The prototypical systems used to study sequential RNA assembly are group II introns, another class of highly-conserved self-splicing ribozymes of biomedical and bioengineering relevance. Group II introns are validated drug targets for antifungal antibiotics, potentially powerful vectors for genetic engineering, and the evolutionary ancestors of the catalytic RNA core of the eukaryotic spliceosome. Integrating single-particle electron cryomicroscopy (cryo-EM), image processing, in solution small-angle X-ray scattering (SAXS), EM-driven molecular dynamics (MD) simulations, structure-based mutagenesis, and enzymatic assays, we have visualized the sequential multidomain assembly of a self-splicing ribozyme of biomedical and bioengineering significance. Our work reveals a distinct dynamic interplay of helical subdomains in the ribozyme’s 5’-terminal scaffold, which acts as a gate to control the docking of 3’-terminal domains.

D Density of the “fully open” state of D1-3 at 4.04 Å resolution. The other conformation, hereafter referred to as the “fully open” state, displays an even larger separation between D1c and i1-i2, a weak density for the ‘peripheral D1c’ motif, and disordered Z-anchor and θ nucleotides, which engage in tertiary contacts between D1 and D2. Analogously, in the D1-3 dataset, we can observe density for D2 in the “partly open”, but not in the “fully open” states. Moreover, we cannot observe density for D3 in either of the two states. In the “fully open” state of D1-3, though, both A72 and C116 orients towards the core of the D1c helix, as in the “catalytic” state. In this “intermediate” state, residue U13 plays a crucial role by replacing residue A12, forming a stacking interaction with A110. Finally, in the “fully open” structure, the stacking interaction between U13 and A110 is maintained. More quantitatively, from our free energy surface (FES) estimation, the “partly open” state is the deepest energy minimum, ~2 kcal•mol−1 lower in energy than the “fully open” state, passing through a metastable “intermediate” state, ~4 kcal•mol−1 higher than the “partly open”. Furthermore, ‘angle A’ progressively increases from 65.8° for sub-state model 1 to 80.5° for sub-state model 20 for the D1-2 dataset, and from 66.9° for sub-state model 1 to 75.1° for sub-state model 20 for the D1-3 dataset, respectively. Finally, the ‘gate distance’ progressively increases from 33.8 Å for sub-state model 1 to 37.8 Å for sub-state model 20 for the D1-2 dataset, and from 34.6 Å for sub-state model 1 to 36.5 Å for sub-state model 20 for the D1-3 dataset, respectively.

> GGGUUAUGUGUGCCCGGCAUGGGUGCAGUCUAUAGGGUGAGAGUCCCGAACUGUGAAGGCAGAAGUAACAGUUAGCCUAACGCAAGGGUGUCCGUGGCGACAUGGAAUCUGAAGGAAGCGGACGGCAAACCUUCGGUCUGAGGAACACGAACUUCAUAUGAGGCUAGGUAUCAAUGGAUGAGUUUGCAUAACAAAACAAAGUCCUUUCUGCCAAAGUUGGUACAGAGUAAAUGAAGCAGAUUGAUGAAGGGAAAGACUGCAUUCUUACCCGGGGAGGUCUGGAAACAGAAGUCAGCAGAAGUCAUAGUACCCUGUUCGCAGGGGAAGGACGGAA N-{5-[(3R)-3-{[5-(acetylamino)-1,3,4-thiadiazol-2-yl]amino}pyrrolidin-1-yl]-1,3,4-thiadiazol-2-yl}acetamide | C12 H16 N8 O2 S2 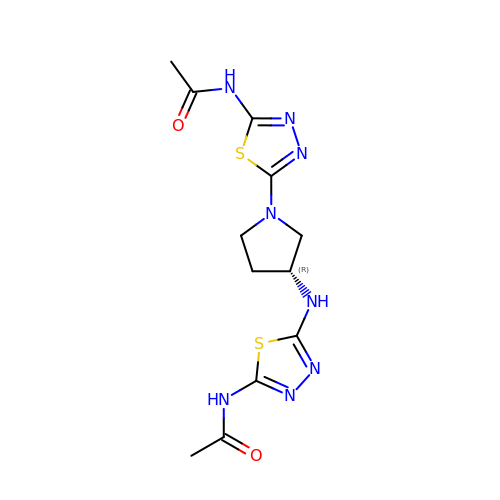| YVDVVIJXVARLFM-MRVPVSSYSA-N>[4x]MFEQRV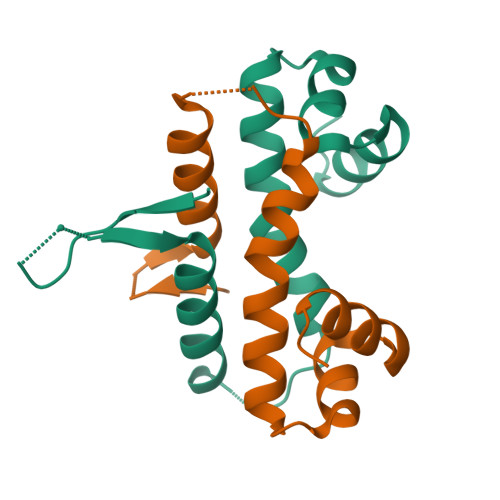NSDVLTVSTVNSQDQVTQKPLRDSVKQALKNYFAQLNGQDVNDLYELVLAEVEQPLLDMVMQYTYGNQTRAALMMGINRGTLRKKLKKYGMN>GMHVDIELPLGRATALQ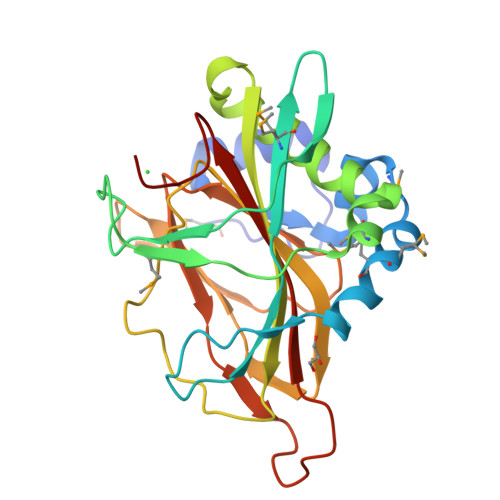RLRAQGFCVLTPAALETLTGMPLDAFDMMLPYWEELAPDLHLKDGGHYRYRRHGCFMQTLQPGQLETVQHRAHWQPTTYNALHGGMERWFEPLSNEMIHLPSWSALLVALGELFAKLRAPQGGRWYIEAHPFRIDTEGGVGRPTPEGAHRDGVDFVAVVFIGRQGVRGGETRVFDAAGPQGVRFTLEQPWTVLLLDDQQVIHESTPLLPLDPADPAVPAHRDTLVLTYRSGGFQAPA[2x]>TCGGCGCC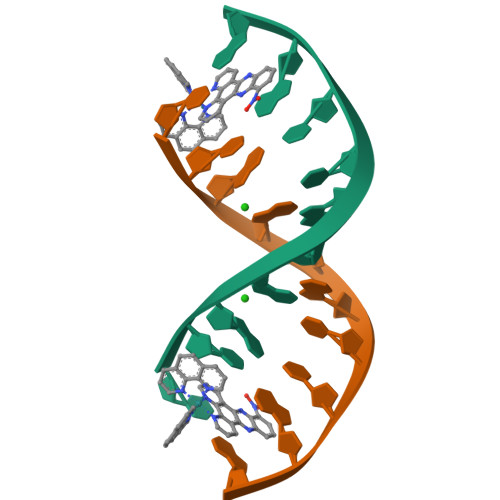GA[2x]>SNAMMSTHYIAGQWLAGQGETLESLDPVGQGVVWSGRGADATQVDAAVCAAREAFPAWARRPLEQRIELLERFAATLKSRADELARVIGEETGKPLWESATEVTSMVNKVAISVQAFRERTGEKSGPLADATAVLRHKPHGVVAVFGPYNFPGHLPNGHIVPALLAGNCVVFKPSELTPKVAELTLKAWIQAGLPAGVLNLVQGGRETGVALAAHRGLDGLFFTGSSRTGNLLHSQFGGQPQKILALEMGGNNPLVVEEVADLDAAVYTIIQSAFISAGQRCTCARRLLVPQGAWGDALLARLVAVSATLRVGRFDEQPAPFMGAVISLSAAEHLLKAQEHLIGKGAQPLLAMTQPIDGAALLTPGILDVSAVAERPDEEFFGPLLQVIRYSDFAAAIREANATQY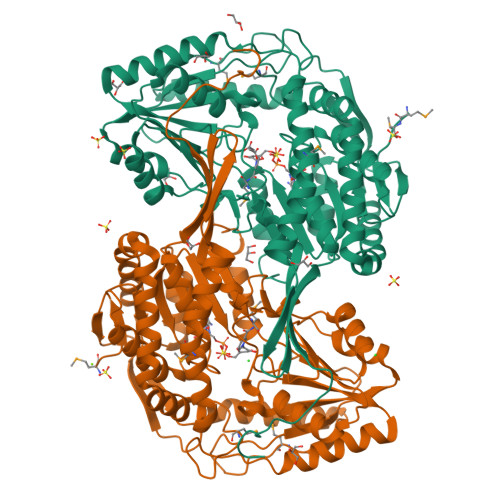GLAAGLLSDSRERFEQFLVESRAGIVNWNKQLTGAASSAPFGGIGASGNHRPSAYYAADYCAYPVASLESPSVSLPATLTPGIS[2x]>[6x]MKLITAIVKPF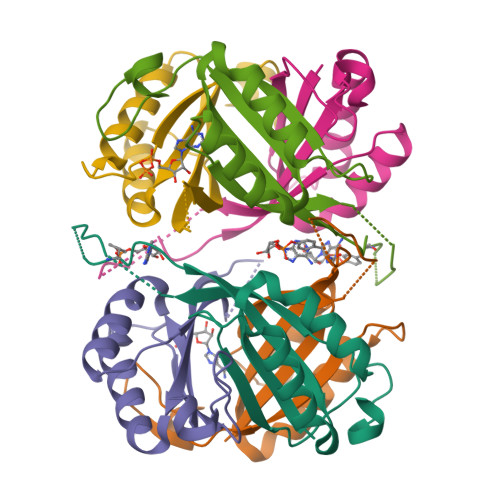TLTDIKDALEQAGVQGMTVTETQGFGQQKGHTEVYRGAEYAVDFVPKVKIEVIISDAQAEEVINIIVETARTGKVGDGKVWMTNIEELVRVRTGERGEAAL>MEFFGETWRRELAAEFEKPYFKQLMSFVADERSRHTVYPPADQVYSWTEMCDIQDVKVVILGQDPYHGPNQAHGLCFSVQKPVPPPPSLVNIYKELCTDIDGFKHPGHGDLSGWAKQGVLLLNAVLTVRAHQANSHKDRGWETFTDAVIKWLSVNREGVVFLLWGSYAHKKGATIDRKRHHVLQAVHPSPLSAHRGFLGCKHFSKANGLLKLSGTEPINWRAL[8x];>MTNLSDIIEKETGKQLVIQESILMLPEEVEEVIGNKPESDILVHTAYDESTDENVMLLTSDAPEYKPWALVIQDSNGENKIKML[8x]

Uracil-DNA N-glycosylase (UNG) is a DNA-repair enzyme which initiates the removal of uracil in the base-excision repair (BER) pathway by cleaving the N-glycosidic bond between the uracil and the deoxyribose backbone. Uracil-DNA N-glycosylase from Atlantic cod (cUNG) shows cold-adapted features such as high catalytic efficiency, a low temperature optimum for activity and reduced thermal stability compared with its mesophilic homologue human UNG (hUNG). Ugi is a small (9.5 kDa), acidic (pI 4.2) and heat-resistant protein encoded by the Bacillus subtillis bacteriophages (PBS1 and PBS2), which use uracil instead of thymine as a normal component of their DNA. It blocks access to the active site of UNG by inserting its β1 strand into the conserved DNA-binding groove of the enzyme without contacting the uracil-specificity pocket.

The crystal structure of the cUNG–Ugi complex was determined to 1.9 Å resolution with eight cUNG–Ugi complexes in the asymmetric unit, all related by non­crystallographic symmetry. However, the crystal structure of the cUNG–Ugi complex reveals that the conformation of cUNG is almost identical to the uncomplexed cUNG structure. The largest differences are found in the Ugi molecules, which are very flexible in some loop areas not involved in complex formation (loops 29–35, 48–53 and 74–78), especially in loop 29–35, which has poor electron density and large B factors. According to the analysis, the interface area in cUNG–Ugi (average value of 1043 Å2) is smaller than that in hUNG–Ugi (1093 Å2). The interface analysis also shows that the average hydrogen-bond distances are slightly shorter in the cUNG–Ugi structure (2.8 Å compared with 2.9 Å in hUNG) even though most hydrogen bonds are formed between the same residues as in hUNG–Ugi. There also seems to be more alternative hydrogen bonds and side chain-to-main chain hydrogen bonds in cUNG–Ugi, as well as two electrostatic interactions in the cUNG–Ugi interface (Lys218–Asp40 and His250–Glu28) which are not found in hUNG–Ugi. For example, both the DNA backbone phosphate-mimicking Ugi residues (Glu20 in the inserted β-sheet and Glu28 in the following α-helix) are bound tightly in cUNG–Ugi. In particular, the Glu171Val, Val185Lys, Gln250His and Tyr275His substitutions in cUNG compared with hUNG result in more favourable interactions with the negatively charged Ugi and the DNA substrate. The larger binding enthalpy of cUNG–Ugi (−25.1 kJ mol−1 at 25°C compared with −9.4 kJ mol−1 for hUNG–Ugi) clearly indicates that the electrostatic inter­actions in cUNG–Ugi are more stabilizing than those found in the hUNG–Ugi complex. The co-crystal structure of cUNG–Ugi presented in this study supports the previously reported DNA-mimicking properties of Ugi.>RAPDSVDYRKKGYVTPVKNQGQCGSCWAFSSVGALEGQLKKKTGKLLNLSPQNLVDCVSENDGCGGGYMTNAFQYVQKNRGIDSEDAYPYVGQEESCMYNPTGKAAKCRGYREIPEGNEKALKRAVARVGPVSVAIDASLTSFQFYSKGVYYDESCNSDNLNHAVLAVGYGIQKGNKHWIIKNSWGENWGNKGYILMARN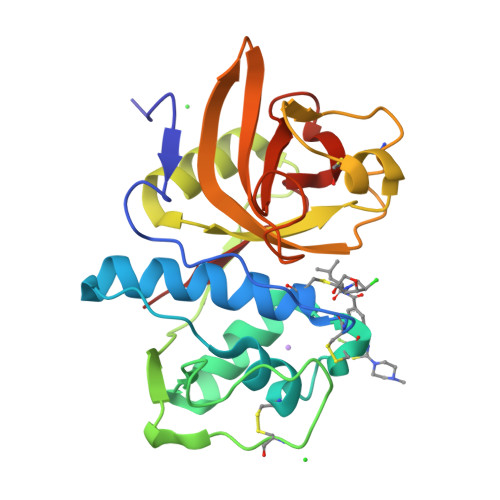KNNACGIANLASFPKM[4x]>MTSENPLLALREKISALDEKLLALFAERRELAVEVGKAKLLSHRPVRDIDRERDLLERLITLGKAHHLDAHFITRTFQLGIEYSVLTQQALLE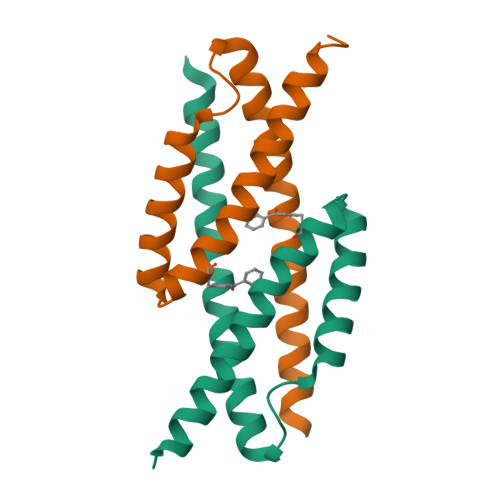HHHHHH[2x]Here we report a functional and structural genomics effort that applied saturation-level transposon mutagenesis and next generation sequencing (Tn-seq) to identify essential genes in B. thailandensis, followed by high-throughput structure determination. We used an “ortholog rescue” approach to maximize structural coverage of these gene families, which are likely to be essential not only in B. thailandensis, but also in related, but more virulent, Burkholderia species, such as B. pseudomallei. Using only seven Burkholderia species to select orthologs of essential genes, we solved structures for 49/406 essential gene families, and for 56 total Burkholderia protein targets (including seven ortholog replicates). Of these 56 targets, 25 satisfied criteria for being a potential antimicrobial drug target.

One strategy that has been employed to improve success rates is to “rescue” such proteins by adding orthologs from related species to the pipeline, based on the assumptions that many of these will have slightly different physical properties that may improve their solubility or crystallization, and that close orthologs will have structures sufficiently similar to the original target to be useful as surrogates in drug design. By using an ortholog rescue strategy for insoluble or difficult to crystallize targets, we increased our structural coverage of B. thailandensis essential genes from 31/406 (7.6%) to 49/406 (12.1%).

>[2x]GPGSMSGIDPKRFGKVAVLFGGESAEREVSLTSGRLVLQGLRDAGIDAHPFDPAERPLSALKDEGFVRAFNALHGGYGENGQIQGALDFYGIRYTGSGVLGSALGLDKFRTKLVWQQTGVPTPPFETVMRGDDYAARATDIVAKLGLPLFVKPASEGSSVAVLKVKTADALPAALSEAATHDKIVIVEKSIEGGGEYTACIAGDLDLPLIKIVPAGEFYDYHAKYVANDTQYLIPCGLPAEQETELKRIARRAFDVLGCTDWGRADFMLDAAGNAYFLEVNTAPGMTDHSLPPKAARSIGIGYSELVVKVLSLTLND>SNAMRAYFEYRHLVTFADTNLVGNVYFTNYLSWQGACRERFLAEKAPKTVARMHDDLALVTSSCSCEFFSELYALDTVSVRMSLVGIDFHQITMGFEYYRVTDGPARLVARGEQTVACTLRAEDGLT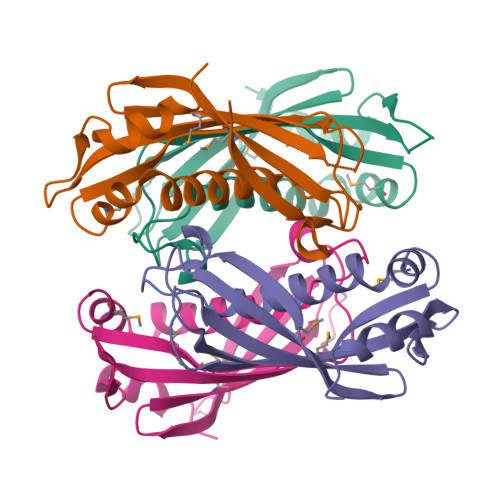PVEVPDELRTALDAYAPDPHGALRPRSETPPR[12x]> MSSGAGSDATGAGGVHAA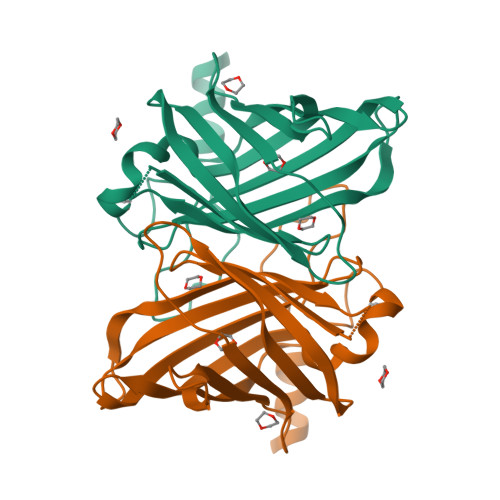GSGDRAVAAAVERAKATAARNIPAFDDLPVPADTANLREGADLNNALLALLPLVGVWRGEGEGRGPDGDYRFGQQIVVSHDGGDYLNWESRSWRLTATGDYQEPGLREAGFWRFVADPYDPSESQAIELLLAHSAGYVELFYGRPRTQSSWELVTDALARSRSGVLVGGAKRLYGIVEGGDLAYVEERVDADGGLVPHLSARLSRFVG> MEEQPQMQDADEPADSGGEGRAGGPPQVAGAQAACSEDRMTLLLRLRAQTKQQLLEYKSMVDASEEKTPEQIMQEKQIEAKIEDLENEIEEVKVAFEIKKLALDRMRLSTALKKNLEKISRQSSVLMDNMKHLLELNKLIMKSQQESWDLEEKLLDIRKKRLQLKQASESKLLEIQTEKNKQKIDLDSMENSERI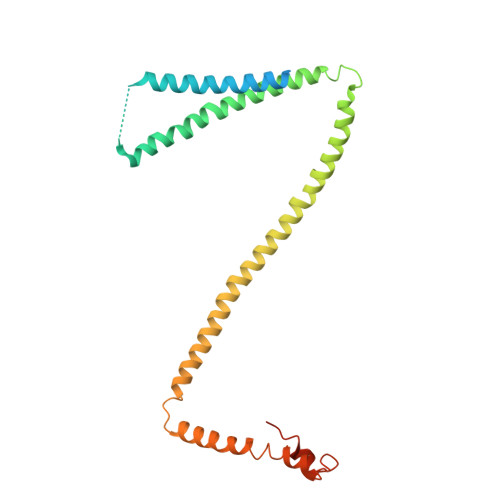KIIRQNLQMEIKITTVIQHVFQNLILGSKVNWAEDPALKEIVLQLEKNVDMMHHHHHH>[5x]QTDMSRKAFVFPKESDTSYVSLKAPLTKPLKAFTVCLHFYTELSSTRGYSIFSYATKRQDNEILIFWSKDIGYSFTVGGSEILFEVPEVTVAPVHICTSWESASGIVEFWVDGKPRVRKSLKKGYTVGAEASIILGQEQDSFGGNFEGSQSLVGDIGNVNMWDFVLSPDEINTIYLGGPFSPNVLNWRALKYEVQGEVFTKPQLWP

C-reactive protein (CRP) is a pentameric protein of 115 kDa composed of five identical non-covalently associated pentraxin domains. The B-face binds to a range of ligands, with the canonical example being phosphocholine (PCh) head groups in lipids such as phosphatidylcholine. This is a calcium-dependent interaction, with each CRP monomer chelating two adjacent Ca2+ ions. The A-face modulates many effector functions of CRP, such as activation of the classical complement pathway, where binding of complement component C1q to CRP is mediated via predominantly electrostatic interactions between the Ca2+-containing globular head domain of C1q (gC1q) and the A-face of CRP.

Maps corresponding to pentameric CRP were solved with both C1 (no symmetry applied) and C5 symmetry. In all cases, applying C5 symmetry yielded maps of better resolution, corresponding to 3.2 – 3.3 Å. The increase in resolution upon map symmetrisation and high degree of similarity in the resulting maps and models strongly suggests that solution-phase CRP pentamers adopt C5 symmetry, which is reinforced by the low deviation in the angles between subunits in the C1-symmetrised pentameric models. Structural analysis of pentamers strongly suggests that pentameric CRP adopts C5 symmetry in solution. Within the structures obtained by cryoEM, five intersubunit ionic bonds contribute to monomer-monomer interactions within the pentamer. These bonds form an ionic zipper from the A-face to the B-face of CRP. One of the salt bridges, Lys123–Glu197, is present at pH 7.5 but absent at pH 5. In agreement with our cryoEM data, Lys123–Glu197 in all crystal structures was shorter than pentameric CRP at pH 5, with an average bond length of 3.0 Å compared to 6.0 Å.N-[8-(cyclohexyloxy)-1-oxo-2-phenyl-1H-pyrido[2,1-b][1,3]benzothiazole-4-carbonyl]-L-tyrosine | C33 H30 N2 O6 S | 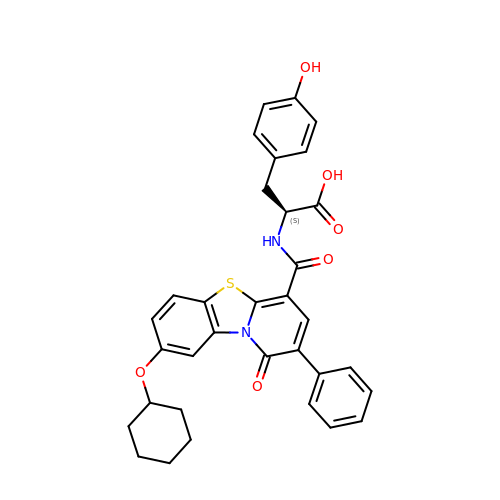PTUWWNGMUPSKDC-MHZLTWQESA-N> MNGSPPVIGGSSGGVGPMIVELPLEKIRRPLMRTRSNDQNKVKELMDSIRQIG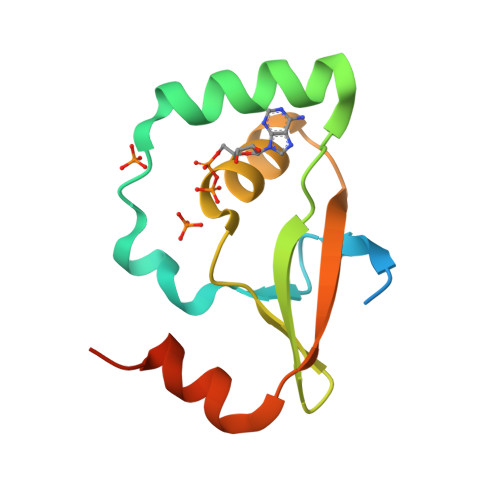LQVPIDVIEVDGTYYGFSGCHRYEAHQKLGLPTIRCKIRKGTKETLRHHLRLEHHHHHH>[5x]MTVTYTARVAKARFGGFSKLLLLWRGSIYKLLWRELLCFLGLFMALSAAYRFVLTEEQKRYFEKLVLYCDRYASLIPVSFVLGFYVTLVVHRWWNQYLSMPLTDALMCVVVGTVHGHDERGRLYRRTLMRYAGLSGVLILRSVSTAVFKRFPTIDHVVEAGFMTREERKKFENLNSSYNKYWVPCVWFCNLAAQAR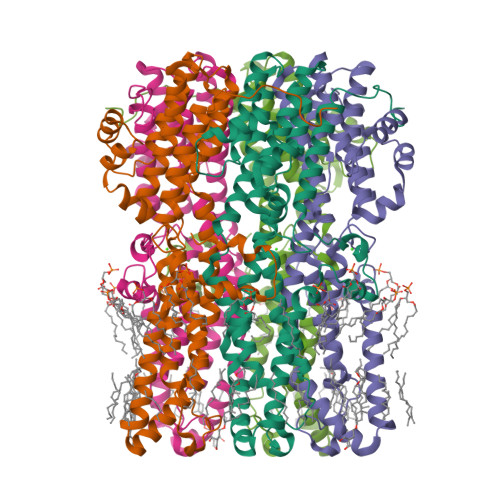REGRIRDNGAFKLLLEELNVFRSKCGMLFHYDWISVPLVYTQVVTIAVYSYFLACLIGRQFLDPAQGYKDHDLDLCVPIFTLLQFFFYAGWLKVAEQLINPFGEDDDDFETNFLIDRCFQVSMLAVDEMYDDLAMLEKDLYWDAAEARA> MENTENSVDSKSIKNLEPKIIHGSESMDSGISLDNSYKMDYPEMGLCIIINNKNFHKSTGMTSRSGTDVDAANLRETFRNLKYEVRNKNDLTREEIVELMRDVSKEDHSKR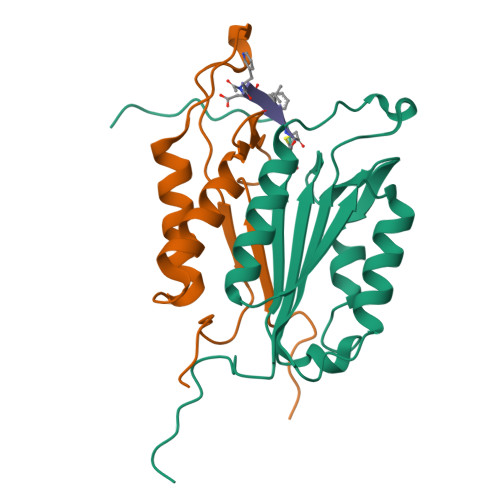SSFVCVLLSHGEEGIIFGTNGPVDLKKITNFFRGDRCRSLTGKPKLFIIQACRGTELDCGIETD;> SGVDDDMACHKIPVEADFLYAYSTAPGYYSWRNSKDGSWFIQSLCAMLKQYADKLEFMHILTRVNRKVATEFESFSFDATFHAKKQIPCIVSMLTKELYFYHLEHHHHHH The rational design of small molecules that target specific DNA sequences is a promising strategy to modulate gene expression. This report focuses on a diamidinobenzimidazole compound, whose selective binding to the minor groove of AT DNA sequences holds broad significance in the molecular recognition of AT-rich human promoter sequences. The specialized method of X-ray crystallography was utilized to investigate how the sequence-dependent recognition properties in general, A-tract, and alternating AT sequences affect the binding of diamidinobenzimidazole in the DNA minor groove. A strong and direct hydrogen bond between the N-H of the benzimidazole and an H-bond acceptor atom in the minor groove is essential for DNA recognition in all sequences described. In addition, the diamidine compound specifically utilizes an interfacial water molecule for its DNA binding.

The A4-DB1476 complex structure is reported at 1.55 Å, with Rwork and Rfree at 22.0 and 24.7%, respectively. The minor groove binder, DB1476, binds to the asymmetric A4-DNA sequence in a singular orientation. The presence of stabilizing external water, like in the −A3T3– and −ATAT– sequences, necessitates the selection of a favored orientation of DB1476. The described prominent features of DB1476 like the BI-N-H bifurcated hydrogen bonding and the strong direct hydrogen at one amidine (C-N4) remain consistent in the binding of the A4-DNA minor groove. The amidine A-N6 has a bonding distance of 3.6 Å from the DNA, suggesting the presence of water-assisted hydrogen bonding, which is expected from the curvature of the ligand. However, from the structure, the waters in the region appear too dynamic to be observed from the X-ray structure. Nonetheless, the presence of an extensive water network across the minor groove stabilizes the A4 complex relatively well (KD = 15 nM). The A4-DB1476 complex structure shows similarity with the AATT-DB1476-II structure in that DB1476 binding extends outside the AT-tract (C-N4 bond with C9). A bifurcated hydrogen bonding, a strong direct H-bond, and an amidine terminal water network stabilize both structures. This suggests the asymmetric A4 DNA, compared to the symmetric AATT, has not caused any notable change in the AT recognition by DB1476 and the overall DNA global structure.

> CGCGAAAACGCG;> CGCGTTTTCGCG> MAHHHHHHMALVELKVPDIGGHENVDIIAVEVNVGDTIAVDDTLITLETDKATMDVPAEVAGVIKEVKVKVGDKISEGGLIVVVEAEGAAAAPKAEAAAAPAQEAPKAAAPAPQAAQFGGAADAEYDVVVLGGGPGGYSAAFAAADEGLKVAIVERYKTLGGVCLNVGCIPSKALLHNAAVIDEVRHLAANGIKYPEPELDIDMLRAYKDGVVSRLTGGLAGMAKSRKVDVIQGDGQFLDPHHLEVSLTAGDAYEQAAPTGEKKIVAFKNCIIAAGSRVTKLPFIPEDPRIIDSSGALALKEVPGKLLIIGGGIIGLEMGTVYSTLGSRLDVVEMMDGLMQGADRDLVKVWQKQNEYRFDNIMVNTKTVAVEPKEDGVYVTFEGANAPKEPQRYDAVLVAAGRAPNGKL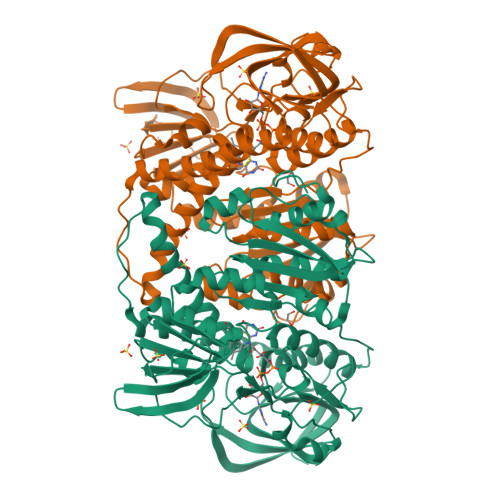ISAEKAGVAVTDRGFIEVDKQMRTNVPHIYAIGDIVGQPMLAHKAVHEGHVAAENCAGHKAYFDARVIPGVAYTSPEVAWVGETELSAKASGRKITKANFPWAASGRAIANGCDNGFTKLIFDAETGRIIGGGIVGPNGGDMIGEVCLAIEMGCDAADIGKTIHPHPTLGESIGMAAEVALGVCTDLPPQKKK>[2x]SQAARVDYIAPWWVVWLHSVPHVGLRLQPVNSTFSPGDESYQESLLFLGLVAAVCLGLNLIFLVAYLVCACHCRRDDAVQTKQHHSCCITWTAVVAGLICCAAVGVGFYGNSETNDGAYQLMYSLDDANHTFSGIDALVSGTTQKMKVDLEQHLARLSEIFAARGDYLQTLKFIQQMAGSVVVQLSGLPVWREVTMELTKLSDQTGYVEYYRWLSYLLLFILDLVICLIACLGLAKRSKCLLASML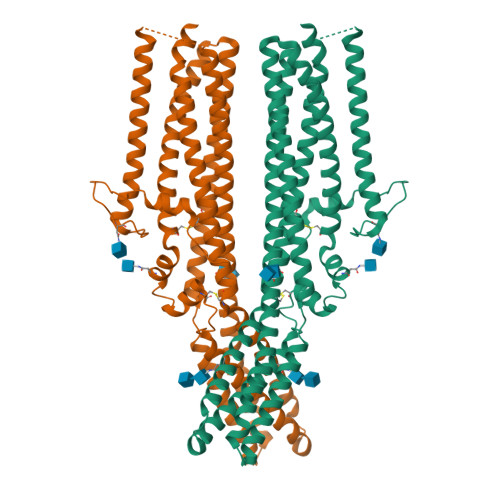CCGALSLLLSWASLAADGSAAVATSDFCVAPDTFILNVTEGQISTEVTRYYLYCSQSGSSPFQQTLTTFQRALTTMQIQVAGLLQFAVPLFSTAEEDLLAIQLLLNSSESSLHQLTAMVDCRGLHKDYLDALAGICYDGLQGLLYLGLFSFLAALAFSTMICAGPRAWKHFTTRNRDYDDIDDDDPFNPQAWRMAAHSPPRGQLHSFCSYSSGLGSQTSLQPPAQTISNAPVSEYMNQAMLFGRNPRYENVPLIGRASPPPTYSPSMRATYLSVADEHLRHYGNQFPAALEVLFQ>MILIADSGSTKTHWNVLDQGRVIGEIFTKGMNPFFQTPEEMGREIERTLLPQLNSNRFCEVHFFGAGCIPEKVPVVRNVLKGCLDVSSLIEVDTDMLAAAKASCGRSPGIVCIMGTGSNSCFYDGEKIAANVSPLGFILGDEGSGAVLGKLLIGDLLKNQMGEELKEKFLRQYELTPANIIERVYRQPFPNRFLAGISPFLAENIEHPAIHSLVLNAFKSFLTRNVMQFDYTRYKAHFIGSVAYYYKDILEEAAAATGIRTGTIVRNPMEGLRTYYSTVAKTV[4x]

Unlike other bacteria, the pathogenic Tannerella forsythia, a member of the red complex group of bacteria associated with the late stages of periodontitis, lacks biosynthetic pathways for MurNAc production and therefore obtains MurNAc from the environment. Sugar kinases play a crucial role in the MurNAc recycling process, activating the sugar molecules by phosphorylation. MurK and K1058 are two sugar kinases of the cell wall recycling system of T. forsythia, sharing a sequence identity of 44% and separated by a single PGN-scavenging operon within the genome. Structural and sequence data showed that MurK and K1058 both belong to the group of ribonuclease H-like kinases and are members of the ASKHA (acetate and sugar kinase/hsc70/actin) superfamily.

We obtained triclinic crystals for MurK (termed MurKapo), which contain four protomers in the asymmetric unit (ASU) that form two biological dimers. A detailed Cα-RMSD analysis of all four chains in MurKapo showed that both protomers of a dimer possess a virtually identical conformation that is slightly different to the second dimer of the ASU. The dimerization interface of the apo enzyme buries a surface of around 1160 Å2 and involves just two residues (F34 and F35) of the N-terminal domain, whereas all other contacts to the adjacent protomer were made by several locations on the α-helical insertion of the C-terminal domain. These include residues in the helices α4-α9 and the loop region in between β8 and α4, as well as residues in the loop region α10 to β9. Soaking experiments with MurKapo crystals using MurNAc failed, probably due to a rearrangement of the N-terminal domain upon substrate uptake ultimately leading to severe crystal damage. The induced fit of MurK can be visualized by superposing the C-terminal domain of the unliganded MurKapo (“open” conformation) to its corresponding C-terminal domain of MurK/MurNAc (“closed” conformation). The best fit utilizes residue range 106 to 266 and results in a Cα-RMSD value of 0.67 Å for 152 aligned residues, showing virtually identical backbone conformation of all the aligned residues of that domain. In the open state, the adjacent protomer does not contribute to the neighboring active site, but the induced fit accompanying the MurNAc uptake enhances the reshaping of the active site by rigidifying the dimeric interface with additional contacts from the N-terminal protomer.>[10x]MAQSSNSTHEPLEVLKEETVNRHR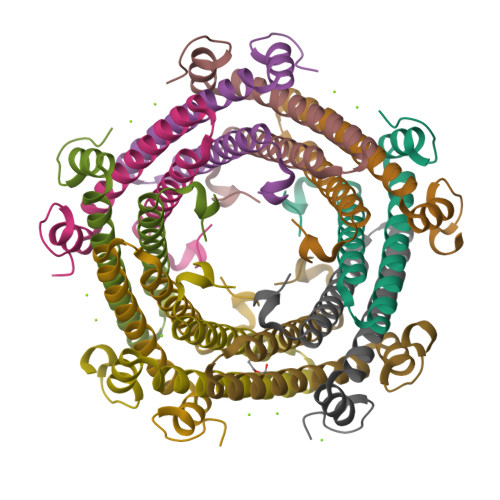AIVSVMEALEAVDWYDQRVDASTDPELTAILAHNRDEAKEAAAMTLEWLRRNDAKWAEHLRTYLFTEGPITAANSSSVDKLAAALEHHHHHH> GADDVVDSSKSFVMENFSSYHGTKPGYVDSIQKGIQKPKSGTQGNYDDDWKGFYSTDNKYDAAGYSVDNENPLSGKAGGVVKVTYPGLTKVLALKVDNAETIKKELGLSLTEPLMEQVGTEEFIKRFGDGASRVVLSLPFAEGSSSVEYINNWEQAKALSVELEINFETRGKRGQDAMYEYMAQACAGNRVRRSVGSSLSCINLDWDVIRDKTKTKIESLKEHGPIKNKMSESPNKTVSEEKAKQYLEEFHQTALEHPELSELKTVTGTNPVFAGANYAAWAVNVAQVIDSETADNLEKTTAALSILPGIGSVMGIADGAVHHNTEEIVAQSIALSSLMVAQAIPLVGELVDIGFAAYNFVESIINLFQVVHNSYNRPAYSPGHKTQPFLHDGYAVSWNTVEDSIIRTGFQGESGHDIKITAENTPLPIAGVLLPTIPGKLDVNKSKTHI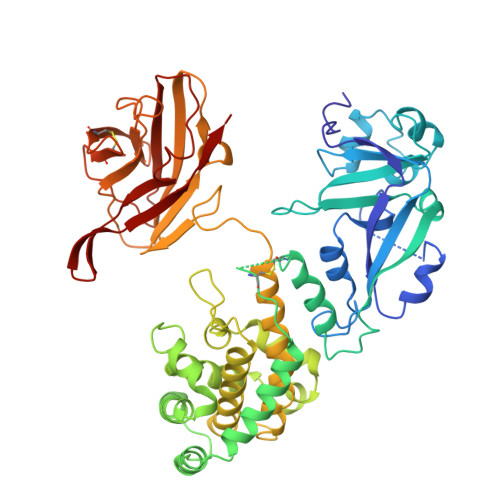SVNGRKIRMRCRAIDGDVTFCRPKSPVYVGNGVHANLHVAFHRSSSEKIHSNEISSDSIGVLGYQKTVDHTKVNSKLSLFFEIKS> MATKQAHKRLTKEYKLMVENPPPYILARPNEDNILEWHYIITGPADTPYKGGQYHGTLTFPSDYPYKPPAIRMITPNG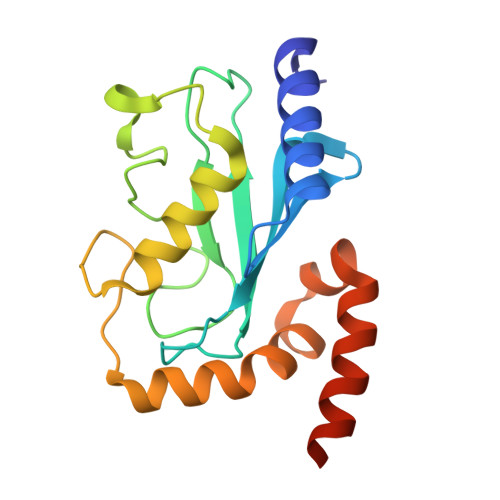RFKPNTRLCLSMSDYHPDTWNPGWSVSTILNGLLSFMTSDEATTGSITTSDHQKKTLARNSISYNTFQNVRFKLIFPEVVQENVETLEKRKLDELPETGG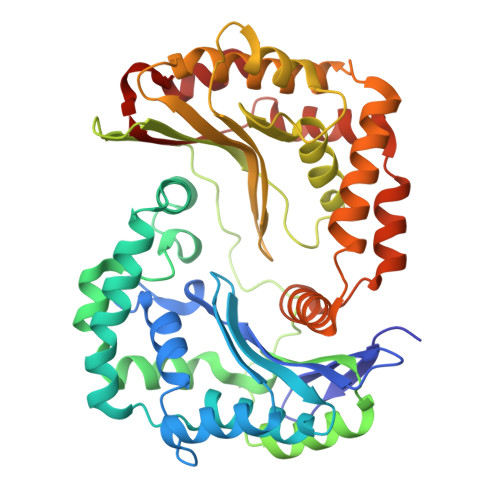> ASQIPGTRTSKLPNGLTIATEYIPNTSSATVGIFVDAGSRAENVKNNGTAHFLEHLAFKGTQNRPQQGIELEIENIGSHLNAYTSRENTVYYAKSLQEDIPKAVDILSDILTKSVLDNSAIERERDVIIRESEEVDKMYDEVVFDHLHEITYKDQPLGRTILGPIKNIKSITRTDLKDYITKNYKGDRMVLAGAGAVDHEKLVQYAQKYFGHVPKSESPVPLGSPRGPLPVFCRGERFIKENTLPTTHIAIALEGVSWSAPDYFVALATQAIVGNWDRAIGTGTNSPSPLAVAASQNGSLANSYMSFSTSYADSGLWGMYIVTDSNEHNVRLIVNEILKEWKRIKSGKISDAEVNRAKAQLKAALLLSLDGSTAIVEDIGRQVVTTGKRLSPEEVFEQVDKITKDDIIMWANYRLQNKPVSMVALGNTSTVPNVSYIEEKLNQ>MKSSHHHHHHENLYFQSNAKEQDLDQLNTLIGIANLKKVLSVWESNKLTNTSEKFWQSVLKENTWILSQIFSNPTVLINDEAYVGGKTVKNDSGKLVDFLYANPFSKDAVLIAIKTPSTPLITPTEYRTGVYSAHKDLTGAVTQVLTYKTTLQREYQNIDYNNYRQGIKTDFDIITPCCVVIAGMFDTLTDTAHRHSFELYRKELKNVTVITFDELFERVKG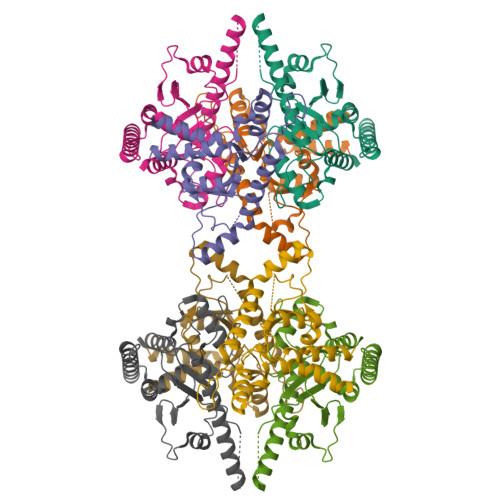LIKLLEG[8x]> SNAMMGIMSDPITILDSSDSLSRLSSESVGRLVVH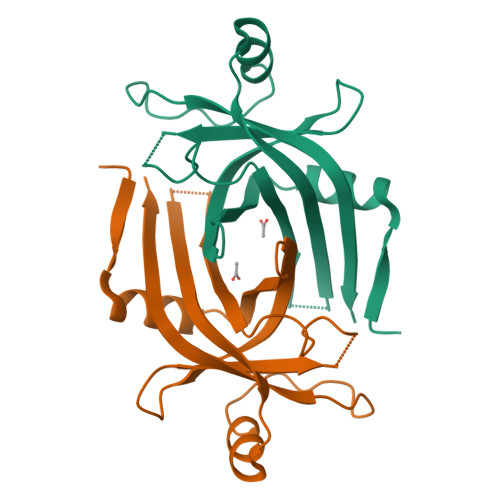RKDDLDIFPVNFVLDYSAEQPRVYFRTAEGTKLFSVNLNSDVLFEVDRFDDAEGWSVVLKGNAYVVRDTEEARHADTLGLKPWLPTLKYNFVRIDVREVSGRAFVFGEEPERY> GSSHHHHHHSSGRENLYFQGHMNGDQNSDVYAQEKQDFVQHFSQIVRVLTEDEMGHPEIGDAIARLKEVLEYNAIGGKYNRGLTVVVAFRELVEPRKQDADSLQRAWTVGWCVELLQAFFLVADDIMDSSLTRRGQICWYQKPGVGLDAINDANLLEACIYRLLKLYCREQPYYLNLIELFLQSSYQTEIGQTLDLLTAPQGNVDLVRFTEKRYKSIVKYKSAFYSFYLPIAAAMYMAG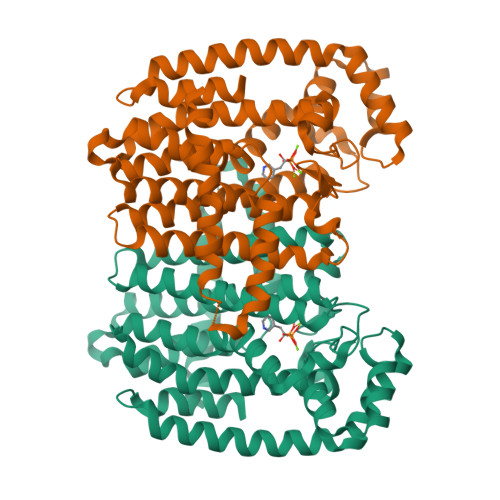IDGEKEHANAKKILLEMGEFFQIQDDYLDLFGDPSVTGKIGTDIQDNKCSWLVVQCLQRATPEQYQILKENYGQKEAEKVARVKALYEELDLPAVFLQYEEDSYSHIMALIEQYAAPLPPAVFLGLARKIYKRRK Voriconazole | C16 H14 F3 N5 O | 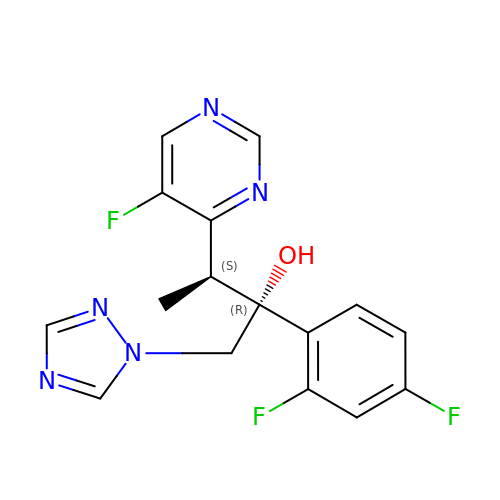BCEHBSKCWLPMDN-MGPLVRAMSA-N Xanthophyllomyces dendrorhous β-fructofuranosidase (Xd-INV, EC 3.2.1.26) is a highly glycosylated dimeric enzyme that belongs to CAZy family GH32 and hydrolyzes sucrose and various fructooligosaccharides (FOS) and fructans releasing fructose. It also catalyzes the synthesis of short-chain FOS, in which the fructosyl moiety is transferred to the sucrose skeleton. Then, crystals from the inactivated pXd-INV-D80A enzyme were used for soaking experiments into β-D-fructose and the different polyphenols tested, to get the corresponding ternary intermediate complexes. All the polyphenolic compounds are bound by stacking their aromatic rings against Trp105, with additional hydrogen bonds from their OH groups to several residues at the active site directly or through several well-ordered water molecules that are linked to the protein.

The transfructosylation rate was 7.4-, 7.8- and 160-fold slower in presence of EGCG, catechol and p-nitrophenol, respectively, compared with the control experiment. Finally, EGGC is accommodated in the catalytic pocket through many atomic interactions. First, the epigallocatechin moiety of EGCG is stacked to Trp105, with the OH next to the Fru O2 being linked to Glu334 carboxylates through water molecules, whilst its second hydroxyl is linked to Gln341(OE1) through a water molecule. The triphenyl ring of epigallocatechin is polar linked to the carbonyl of Leu661 at the C-terminus of the chain. On the other hand, the gallate ring is mainly accommodated by the loop Glu334-Asn342 through direct hydrogen bonds to Gln335 (NE2) and Gln341 (OE1). On the other hand, conformational changes are not observed in the residues at the active site upon binding of the different compounds, with the only exception of a switch in the Glu334 side-chain found in the crystal containing EGGC, possibly due to the steric hindrance associated to this bulky compound. As can be seen, the positions of catechol and the EGCG diphenolic part of benzopirane are very similar, while the aromatic ring of p-nitrophenol is slightly shifted towards the diethylenglycol trapped in the catechol containing crystals. In contrast, catechol/EGCG binding position is shifted from subsite +1 therefore tolerating binding of sucrose donor to a higher extent. In contrast, catechol, HQ, and EGCG bind at the inulin-type subsite +2, occupying the same position that the terminal glucose from 1-kestose. Furthermore, the significant reduction in hydrolysis rate presented with catechol and EGCG may explain the absence of FOS in the first 30–40 minutes of reaction, after which these molecules allow moderate FOS production.

>MVAPLLKTLPFLAAAYAAELDLPNFSALNRRQDNSTSSSAGCSLDQTVAPGNLTLCGNATLFTTFRPKARFIAPEGWMNAPMGLYQRADGSIHAGYQSHPKHIQWGNISQGAAYSSDFTSWTDFNGSEGYKTIWPSQIYDIRGVFDGSIIKEGIDGYPTILYTSTSFGPLGATLNEAEGTETQSLAYTTDDGASWIKLGYGAGQNPVIYEWPETNLTGFRDPYVFQSPRLEALLANTTSITNATGDHFATISGGVHGDGARLFLYRQHTTGEFIKWTYLGPLVTTGYKESYGEWSGNYGINFETAGVTRLNPAGAAWDNGSDTTAVDFVTFGTEQGRADHQNHWPLWAAVDYEVRDNGSIEAVIAYSGVQDWGRSYAYASFPVEGYRQVSVGWIYEDDDNVILAKQFGYQGAFTLFRDLFVKVVENVSPSTPGLFEQASWSTKNSTDGMSVTVTTLGQRVVPETLAAYKGNSTVSTLAPVMLNESAAAYTPFSSQPTDRFYALTGSFEFGLNTTAKAGFRVLASEEEYTDIWFDPASENLTVVRTASSLIKSFGNDTELAKVKLYEIVGAESKTLNLTVFVDGSVIEIYANDEVALSTRAYPWLANSTGAGLLADGTTAGDVVGVSGLELWDGLVDAWPARPANTSQGLVWDGPTAAMYGLFAGY[2x]> MGRLLALVVGAALVSSACGGCVEVDSETEAVYGMTFKILCISCKRRSETNAETFTEWTFRQKGTEEFVKILRYENEVLQLEEDERFEGRVVWNGSRGTKDLQDLSIFITNVTYNHSGDYECHVYRLLFFENYEHNTSVVKKIHIEVVDKANRDMASIVSEIMMYVLIVVLTIWLVAEMIYCYKKIAAATETAAQENASEYLAITSESKENCTGVQVAE;> MHRDAWLPRPAFSLTGLSLFFSLVPPGRSMEVTVPATLNVLNGSDARLPCTFNSCYTVNHKQFSLNWTYQECNNCSEEMFLQFRMKIINLKLERFQDRVEFSGNPSKYDVSVMLRNVQPEDEGIYNCYIMNPPDRHRGHGKIHLQVLMEEPPERDSTVAVIVGASVGGFLAVVILVLMVVKCVRRKKEQKLSTDDLKTEEEGKTDGEGNPDDGAK;> MAQALLVPPGPESFRLFTRESLAAIEKRAAEEKAKKPKKEQDNDDENKPKPNSDLEAGKNLPFIYGDIPPEMVSEPLEDLDPYYINKKTFIVMNKGKAIFRFSATSALYILTPLNPVRKIAIKILVHSLFSMLIMCTILTNCVFMTLSNPPDWTKNVEYTFTGIYTFESLIKILARGFCLEDFTFLRDPWNWLDFSVIVMAYVTEFVSLGNVSALRTFRVLRALKTISVIPGLKTIVGALIQSVKKLSDVMILTVFCLSVFALIGLQLFMGNLRNKCLQWPPSDSAFETNTTSYFNGTMDSNGTFVNVTMSTFNWKDYIGDDSHFYVLDGQKDPLLCGNGSDAGQCPEGYICVKAGRNPNYGYTSFDTFSWAFLSLFRLMTQDYWENLYQLTLRAAGKTYMIFFVLVIFLGSFYLVNLILAVVAMAYEEQNQATLEEAEQKEAEFQQMLEQLKKQQEEAQAVAAASAASRDFSGIGGLGELLESSSEASKLSSKSAKEWRNRRKKRRQREHLEGNNKGERDSFPKSESEDSVKRSSFLFSMDGNRLTSDKKFCSPHQSLLSIRGSLFSPRRNSKTSIFSFRGRAKDVGSENDFADDEHSTFEDSESRRDSLFVPHRHGERRNSNVSQASMSSRMVPGLPANGKMHSTVDCNGVVSLVGGPSALTSPTGQLPPEGTTTETEVRKRRLSSYQISMEMLEDSSGRQRAVSIASILTNTMEELEESRQKCPPCWYRFANVFLIWDCCDAWLKVKHLVNLIVMDPFVDLAITICIVLNTLFMAMEHYPMTEQFSSVLTVGNLVFTGIFTAEMVLKIIAMDPYYYFQEGWNIFDGIIVSLSLMELGLSNVEGLSVLRSFRLLRVFKLAKSWPTLNMLIKIIGNSVGALGNLTLVLAIIVFIFAVVGMQLFGKSYKECVCKINDDCTLPRWHMNDFFHSFLIVFRVLCGEWIETMWDCMEVAGQTMCLIVFMLVMVIGNLVVLNLFLALLLSSFSSDNLAATDDDNEMNNLQIAVGRMQKGIDYVKNKMRECFQKAFFRK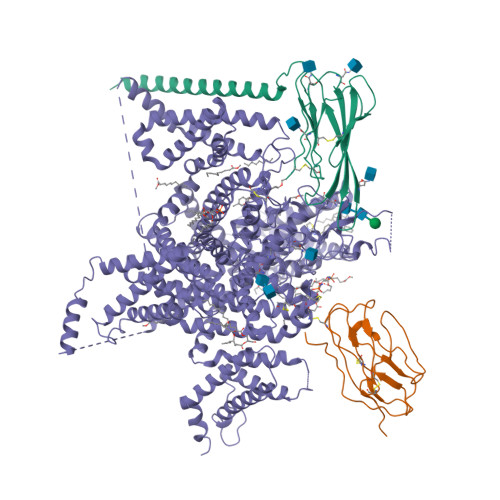PKVIEIHEGNKIDSCMSNNTGIEISKELNYLRDGNGTTSGVGTGSSVEKYVIDENDYMSFINNPSLTVTVPIAVGESDFENLNTEEFSSESELEESKEKLNATSSSEGSTVDVVLPREGEQAETEPEEDLKPEACFTEGCIKKFPFCQVSTEEGKGKIWWNLRKTCYSIVEHNWFETFIVFMILLSSGALAFEDIYIEQRKTIKTMLEYADKVFTYIFILEMLLKWVAYGFQTYFTNAWCWLDFLIVDVSLVSLVANALGYSELGAIKSLRTLRALRPLRALSRFEGMRVVVNALVGAIPSIMNVLLVCLIFWLIFSIMGVNLFAGKFYHCVNMTTGNMFDISDVNNLSDCQALGKQARWKNVKVNFDNVGAGYLALLQVATFKGWMDIMYAAVDSRDVKLQPVYEENLYMYLYFVIFIIFGSFFTLNLFIGVIIDNFNQQKKKFGGQDIFMTEEQKKYYNAMKKLGSKKPQKPIPRPANKFQGMVFDFVTRQVFDISIMILICLNMVTMMVETDDQGKYMTLVLSRINLVFIVLFTGEFVLKLVSLRHYYFTIGWNIFDFVVVILSIVGMFLAEMIEKYFVSPTLFRVIRLARIGRILRLIKGAKGIRTLLFALMMSLPALFNIGLLLFLVMFIYAIFGMSNFAYVKKEAGIDDMFNFETFGNSMICLFQITTSAGWDGLLAPILNSAPPDCDPDTIHPGSSVKGDCGNPSVGIFFFVSYIIISFLVVVNMYIAVILENFSVATEESAEPLSEDDFEMFYEVWEKFDPDATQFIEFSKLSDFAAALDPPLLIAKPNKVQLIAMDLPMVSGDRIHCLDILFAFTKRVLGESGEMDALRIQMEDRFMASNPSKVSYEPITTTLKRKQEEVSAAIIQRNFRCYLLKQRLKNISSNYNKEAIKGRIDLPIKQDMIIDKLNGNSTPEKTDGSSSTTSPPSYDSVTKPDKEKFEKDKPEKESKGKEVRENQK> PISPIETVPVKLKPGMDGPKVKQWPLTEEKIKALVEICTEMEKEGKISKIGPENPYSTPVFAIKKKDSTKWRKLVDFRELNKRTQDFWEVQLGIPHPAGLKKKKSVTVLDVGDAYFSVPLDEDFRKYTAFTIPSINNETPGIRYQYNVLPQGWKGSPAIFQSSMTKIL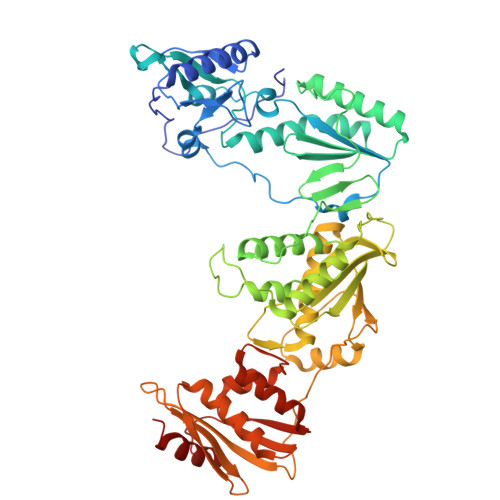EPFKKQNPDIVIYQYMDDLYVGSDLEIGQHRTKIEELRQHLLRWGLTTPDKKHQKEPPLLWMGYELHPDKWTVQPIVLPEKDSWTVNDIQKLVGKLNWASQIYPGIKVRQLCKLLRGTKALTEVIPLTEEAELELAENREILKEPVHGVYYDPSKDLIAEIQKQGQGQWTYQIYQEPFKNLKTGKYARMRGAHTNDVKQLTEAVQKITTESIVIWGKTPKFKLPIQKETWETWWTEYWQATWIPEWEFVNTPPLVKLWYQLEKEPIVGAETFYVDGAANRETKLGKAGYVTNKGRQKVVPLTNTTNQKTQLQAIYLALQDSGLEVNIVTDSQYALGIIQAQPDKSESELVNQIIEQLIKKEKVYLAWVPAHKGIGGNEQVDKLVSAGIRHHHHH> GAMGIAEVQQQLVAAQLAMERDYETQREMETRYRVVLDVSRDPMVLVSMSTGRIVDLNSAAGLLLGGVRQDLLGAAIAQEFEGRRRGEFMETMTNLAATESAAPVEVLARRSQKRLLVVPRVFRAAGERLLLCQIDPAD

The redox-responding transcription factor PpsR (photopigment suppression) from Rhodobacter sphaeroides is such a multi-PAS domain-containing protein. PpsR possesses three PAS domains (designated N-domain, PAS1 and PAS2) and a highly conserved glutamine-rich linker (Q-linker) as well as a C-terminal helix–turn–helix (HTH) DNA-binding motif. PpsR acts as a repressor of photosynthesis and tetrapyrrole-biosynthesis gene expression by binding to palindromic DNA sequences (TGTc-N10-gACA) present in the promoter region of PpsR-regulated genes. Additionally, the function of PpsR is regulated in a blue-light- and oxygen-dependent manner by the antirepressor AppA that, together with PpsR and its cognate DNA, is able to form a light-sensitive ternary AppA–PpsR2–DNA complex.

We finally extended the phases to 1.65 Å resolution using a native data set and refined a high-resolution structure for this variant. The PpsRQ-PAS1 structure revealed a typical PAS fold consisting of a five-stranded antiparallel β-sheet flanked by several helices. In addition to the PAS1 core, part of the Q-­linker adopts an α-helical conformation corresponding to a PAS N-cap. This is important for dimer formation as observed for other N-cap-containing PAS domains. The main dimerization interface is formed by the N-cap, its connecting loop to the PAS core (residues 156–161) and β51. The N-cap further contributes to PpsRQ-PAS1 dimer formation by protecting hydrophobic patches on the PAS core of the symmetry-related molecule, as also reported for a subset of other PAS proteins. The 20 N-­terminal residues are disordered and could not be modelled into the electron-density map. The remaining ordered part of the Q-linker region (residues 143–157) forms a helical element that corresponds to a classical PAS N-cap. As proposed previously, the N-domain also significantly contributes to PpsR oligomer formation and/or integrity, most likely by stabilizing the extended Q-linker helix as shown by the disordered N-terminal Q-linker part of the PpsRQ-PAS1 structure. In contrast to the other studied PpsR variants, PpsRQ-PAS1 exists predominantly as a monomer at the concentrations used in this experiment.>GHMVSRIEQRLIDKGLKVTDQRRVIAQVLSDSADHPDVEEVYRRATAKDPRISIATVYRTVRLFEEESILERHDFGDGRARYEEAPSEHHDHLIDVNSARVIEFTSPEIEALQREIARKHGFRLVGHRLELYGVPLTSGGDSDDK[2x]

In most bacteria, iron homeostasis is regulated primarily by the ferric uptake regulator (Fur). Fur, which was first discovered in Escherichia coli, is a global transcriptional regulator that directly controls the transcription of over 90 genes involved in iron uptake, storage and metabolism. Several holo-Fur structures have been solved, revealing a modular domain organization including an N-terminal DNA-binding domain (DBD) and a C-terminal dimerization domain (DD). In this study, we present six crystal structures of apo-Fur, holo-Fur, Fur in complex with the Fe2+ transport protein (feoAB1) operator and the P. aeruginosa (or E. coli) Fur box.

The sequence in the final co-crystal of the Fur-Mn2+–P. aeruginosa Fur box complex was 5′-CGCGATAATGATAATCATTATCCGC-3′. The functional structure was generated by a crystallographic twofold axis. Surprisingly, binding of two Fur dimers to one dsDNA target site was found in the Fur-Mn2+–P. aeruginosa Fur box structure, with one dimer bound close to the 5′ end of the coding strand and the other dimer close to the 3′ end. The electron density corresponding to the P. aeruginosa Fur box was sufficiently well resolved to allow unambiguous assignment of the DNA nucleotide sequence, except for one missing base at each 3′ end. The two Fur dimers are positioned on almost opposite sides of the double helix, in contrast to the positioning of other prokaryotic helix-turn-helix motif class repressors, such as the trp repressor. In contrast, the two Fur dimers do interact, mostly in the DNA major groove and between the two antiparallel α3 helices of the Fur dimers. There are two hydrogen bonds, two water-mediated hydrogen bonds and two electrostatic interactions at the interface between Glu37, Tyr40, Arg41 and Thr44 of each dimer, suggesting that the inferred cooperativity arises from cross-dimer protein–protein contacts. Arg57 also forms one hydrogen bond with T15′ of the P. aeruginosa Fur box. The negative electrostatic potential in the minor groove of the P. aeruginosa Fur box is enhanced compared with that of the feoAB1 operator, which might further increase the binding ability. Thus, cooperativity can explain why the P. aeruginosa Fur box can tolerate the loss of shape readout by Lys15 when a Fur monomer is positioned at the end of a DNA fragment in the crystal structure.>[2x]MPLD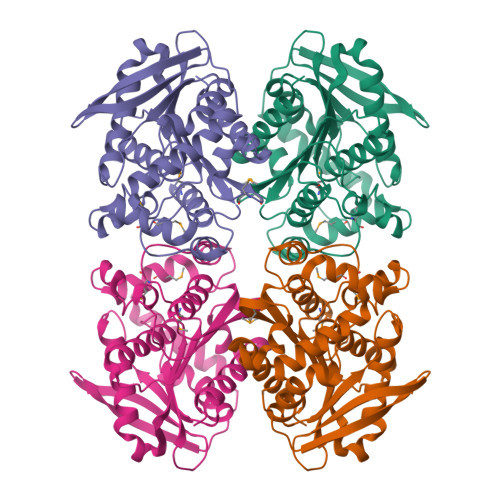PQIKPILERIRALSIAASPQELRRQVEEQSRLLTAAVQEPIAETRDVHIPVSGGSIRARVYFPKKAAGLPAVLYYHGGGFVFGSIETHDHICRRLSRLSDSVVVSVDYRLAPEYKFPTAVEDAYAALKWVADRADELGVDPDRIAVAGDSAGGNLAAVVSILDRNSGEKLVKKQVLIYPVVNMTGVPTASLVEFGVAETTSLPIELMVWFGRQYLKRPEEAYDFKASPLLADLGGLPPALVVTAEYDPLRDEGELYAYKMKASGSRAVAVRFAGMVHGFVSFYPFVDAGREALDLAAASIRSGLQPS>[2x]GPLGSMVSGVGGSGGGRGGGRGGEEEPSSSHTPNNRRGGEQAQSSGTKSLRPRSNTESMSKAIQQYTVDARLHAVFEQSGESGKSFDYSQSLKTTTYGSSVPEQQITAYLSRIQRGGYIQPFGCMIAVDESSFRIIGYSENAREMLGIMPQSVPTLEKPEILAMGTDVRSLFTSSSSILLERAFVAREITLLNPVWIHSKNTGKPFYAILHRIDVGVVIDLEPARTEDPALSIAGAVQSQKLAVRAISQLQALPGGDIKLLCDTVVESVRDLTGYDRVMVHKFHEDEHGEVVAESKRDDLEPYIGLHYPATDIPQASRFLFKQNRVRMIVDCNATPVLVVQDDRLTQSMCLVGSTLRAPHGCHSQYMANMGSIAS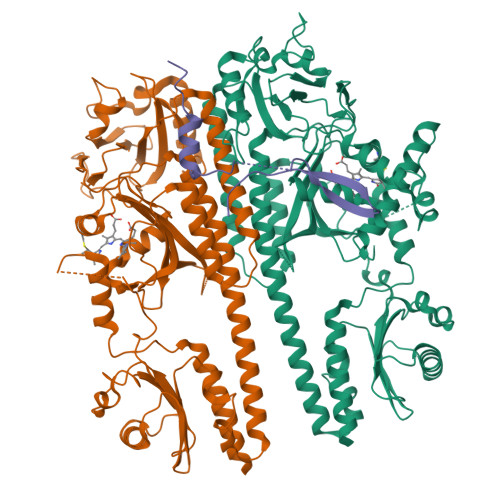LAMAVIINGNEDDGSNVASGRSSMRLWGLVVCHHTSSRCIPFPLRYACEFLMQAFGLQLNMELQLALQMSEKRVLRTQTLLCDMLLRDSPAGIVTQSPSIMDLVKCDGAAFLYHGKYYPLGVAPSEVQIKDVVEWLLANHADSTGLSTDSLGDAGYPGAAALGDAVCGMAVAYITKRDFLFWFRSHTAKEIKWGGAKHHPEDKDDGQRMHPRSSFQAFLEVVKSRSQPWETAEMDAIHSLQLILRDSFKESEAAMNSKVVDGVVQPCRDMAGEQGIDELGAVAREMVRLIETATVPIFAVDAGGCINGWNAKIAELTGLSVEEAMGKSLVSDLIYKENEATVNKLLSRALRGDEEKNVEVKLKTFSPELQGKAVFVVVNACSSKDYLNNIVGVCFVGQDVTSQKIVMDKFINIQGDYKAIVHSPNPLIPPIFAADENTCCLEWNMAMEKLTGWSRSEVIGKMIVGEVFGSCCMLKGPDALTKFMIVLHNAIGGQDTDKFPFPFFDRNGKFVQALLTANKRVSLEGKVIGAFCFLQIPS;> GPLGSMMFLPTDYCCRLSDQEYMELVFENGQILAKGQRSNVSLHNQRTKSIMDLYEAEYNEDFMKSIIHGGGGAITNLGDTQVVPQSHVAAAHETNMLESNKHVD ETHYL 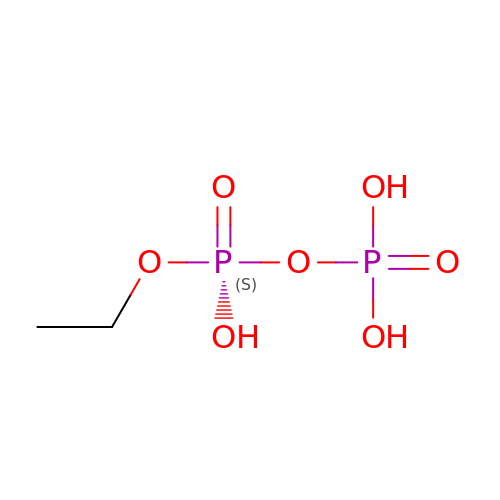DIHYDROGEN DIPHOSPHATE | C2 H8 O7 P2 | OJDJHGIXNZPZFD-UHFFFAOYSA-N>[4x]MIFTKEPANVFYVLVSAFRSNLCDEVNMSRHRHMVSTLRAAPGLYGSVESTDLTGCYREAISSAPTEEKTVRVRCKDKAQALNVARLACNEWEQDCVLVYKSQTHTAGLVYAKGIDGYKAERLPGSFQEVPKGAPLQGCFTIDEFGRRWQVQHHHHHH;>MAKHLFTSESVSEGHPDKIADQISDAVLDAILEQDPKARVACETYVKTGMVLVGGEITTSAWVDIEEITRNTVREIGYVHSDMGFDANSCAVLSAIGKQSPDINQGVDRADPLEQGAGDQGLMFGYATNETDVLMPAPITYAHRLVQRQAEVRKNGTLPWLRPDAKSQVTFQYDDGKIVGIDAVVLSTQHSEEIDQKSLQEAVMEEIIKPILPAEWLTSATKFFINPTGRFVIGGPMGDCGLTGRKIIVDTYGGMARHGGGAFSGKDPSKVDRSAAYAARYVAKNIVAAGLADRCEIQVSYAIGVAEPTSIMVETFGTEKVPSEQLTLLVREFFDLRPYGLIQMLDLLHPIYKETAAYGHFGREHFPWEKTDKAQLLRDAAGLKHHHHHH[8x]

S-Adenosylmethionine lyase (SAMase) of bacteriophage T3 degrades the intracellular SAM pools of the host Escherichia coli cells, thereby inactivating a crucial metabolite involved in a plethora of cellular functions, including DNA methylation. Using single-particle cryoelectron microscopy (cryo-EM) and biochemical assays, we demonstrate that SAMase performs its function by not only degrading SAM but also by interacting with and efficiently inhibiting the host’s methionine S-adenosyltransferase (MAT), the enzyme that produces SAM. E. coli MAT is a dihedral homotetramer (comprised of dimers of dimers) that catalyzes the condensation of ATP and methionine to produce SAM. MAT is an essential enzyme and the only source of SAM in E. coli.

Specifically, SAMase triggers open-ended head-to-tail assembly of E. coli MAT into an unusual linear filamentous structure in which adjacent MAT tetramers are joined by two SAMase dimers. Specifically, each SAMase monomer forms an interaction with a MAT monomer and another SAMase monomer, so that each of the two MAT tetramers are joined in a head-to-tail fashion by two SAMase dimers. The interaction between the adjacent MAT molecules is weak, with an interface of only ∼170 Å. A SAMase monomer is an α/β protein composed of nine antiparallel β-strands forming a barrel-like structure and two helixes positioned outside the barrel. Two T3 SAMase monomers interact along ∼1,000-Å2 isologous interfaces to form a C2-dimer. The MAT-SAMase interface is smaller and occupies ∼600 to 700Å2. The “cracked egg” structure of SAMase dimer pushes one of the two joined MAT tetramers away from the plane. This bend between two adjacent MAT tetramers causes a propagation of right-handed helical twists along the entire SAMase-MAT heteropolymer. However, 6 out of the 21 interface-forming residues, Asp132, Val 133, Ile 178, Ile 211, Ala 214, and Trp 26, are present only in E. coli or in other closely related enteric bacteria. Collectively, DMD simulations together with normal mode analyses suggest that the entrapment of MAT tetramers within the SAMase-mediated filaments leads to an allosteric inhibition of MAT activity via dynamic coupling.> GPGSKTLTRAARDRYAPYFAYAAAQPSDEVTTVRGLSNPLIKTAPVTLPFDLGQAVADNC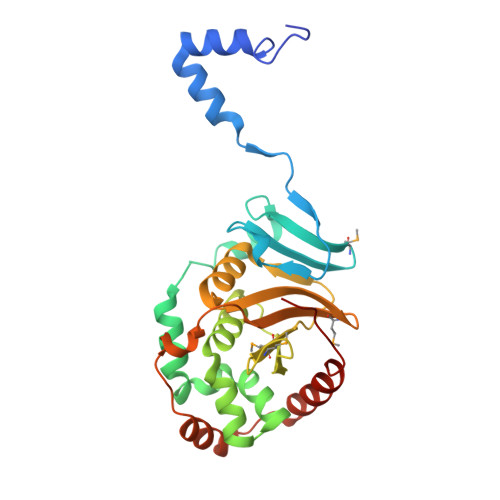LSLSGMGYYLGLGGCCPTCAAAEPRLGRSDRAALVLAYVQQLNSIYEYRVFLASVAARDPSERALEEVLAHPELFFAYYVLRDGGLRDVRVLFFEDPDAQGALMMYVVFPEKSVHVHHRVLDRLLGACAGHRIVAHVWQTMFVLVVRKKGDGRPADDVPAVSASDIYCKMRDISFDGELLLEYKRLYAAFEDFRPPRP>[8x]MIDFGNFYSLIAKNHLSHWLETLPAQIANWQREQQHGLFKQ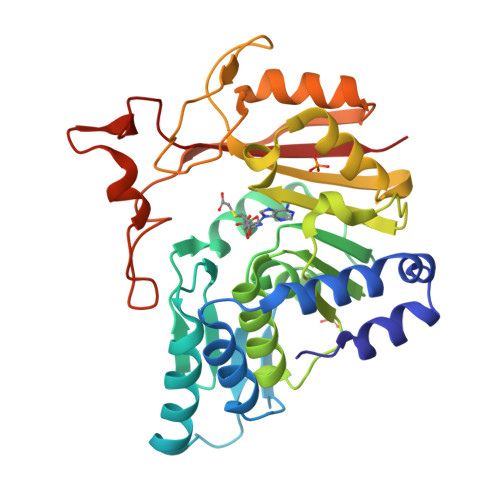WSNAVEFLPEIKPYRLDLLHSVTAESEEPLSAGQIKRIETLMRNLMPWRKGPFSLYGVNIDTEWRSDWKWDRVLPHLSDLTGRTILDVGCGSGYHMWRMIGAGAHLAVGIDPTQLFLCQFEAVRKLLGNDQRAHLLPLGIEQLPALKAFDTVFSMGVLYHRRSPLEHLWQLKDQLVNEGELVLETLVIDGDENTVLVPGDRYAQMRNVYFIPSALALKNWLKKCGFVDIRIADVSVTTTEEQRRTEWMVTESLADFLDPHDPGKTVEGYPAPKRAVLIARKP> MSAKTPLDPALFRPDAISDETRGINDFIIKAFEAVPEWWEIGAATVREARARGEGGFPLPPKSERARTIEIEGKGGHKVPLRIIAPESPKGVYLHIHGGGWVLGACDQQDPMLERIAQNAGLACVSVEYRLAPEHPYPAGPDDCEAAALWLVKNA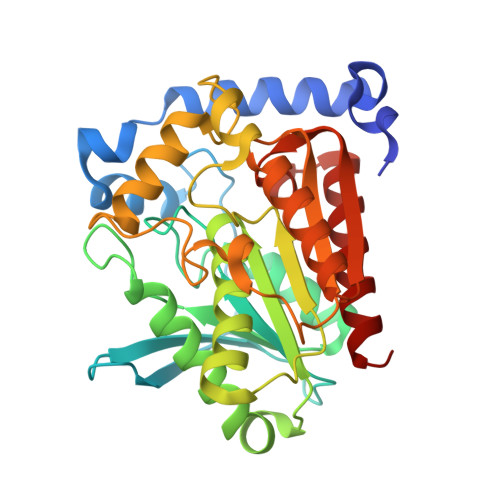KKEFGTEVLTIGGESAGGHLSAVTLLRMRDRHGYKGFKGANLVFGAFDMSMSPSQRVFGNERLVLRTVDIQKFGDAFLPNGEDRRDPDISPLYANLHDMPPALFTVGTRDALVDDTLFMHARWIAAGNEAELGVFPGGAHGFVAFPGEIARAANAQADAFLRRVTGQ> SS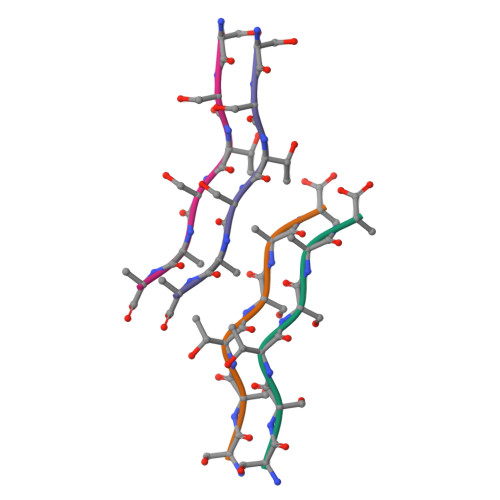TSAA>[2x]DQSDPEDVGKMTTENNIVVDKSDLIPKVLT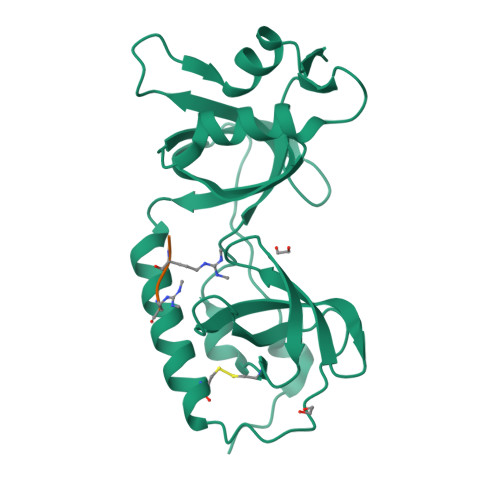LNVGDEFCGVVAHIQTPEDFFCQQLQSGRKLAELQASLSKYCDQLPPRSDFYPAIGDICCAQFSEDDQWYRASVLAYASEESVLVGYVDYGNFEILSLMRLCPIIPKLLELPMQAIKCVLAGVKPSLGIWTPEAICLMKKLVQNKIITVKVVDKLENSSLVELIDKSETPHVSVSKVLLDAGFAVGEQSM;> SSGPARGRGRHPGKGVK> MHHHHHHMPIIEQVRAREILDSRGNPTVEVEVALIDGTFARAAVPSGASTGEHEAVELRDGGDRYGGKGVQKAVQAVLDEIGPAVIGLNADDQRLVDQALVDLDGTPDKSRLGGNAILGVSLAVAKAAADSAELPLFRYVGGPNAHILPVPMMNILNGGAHADTAVDIQEFMVAPIGAPSFVEALRWGAEVYHALKSVLKKEGLSTGLGDEGGFAPDVAGTTAALDLISRAIESAGLRPGADVALALDAAATEFFTDGTGYVFEGTTRTADQMTEFYAGLLGAYPLVSIEDPLSEDDWDGWAALTASIGDRVQIVGDDIFVTNPERLEEGIERGVANALLVKVNQIGTLTETLDAVTLAHHGGYRTMISHRSGETEDTMIADLAVAIGSGQIKTGAPARSERVAKYNQLLRI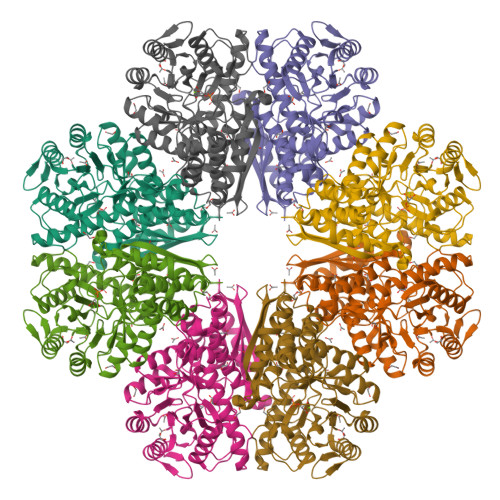EEALGDAARYAGDLAFPRFACETK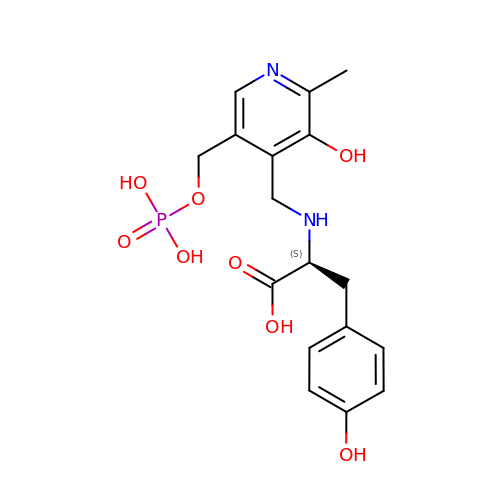N-({3-hydroxy-2-methyl-5-[(phosphonooxy)methyl]pyridin-4-yl}methyl)-L-tyrosine | C17 H21 N2 O8 P | AGEIFYRIXWJCET-HNNXBMFYSA-N({[(2S)-1-(4-amino-2-oxopyrimidin-1(2H)-yl)-3-hydroxypropan-2-yl]oxy}methyl)phosphonic acid | C8 H14 N3 O6 P | 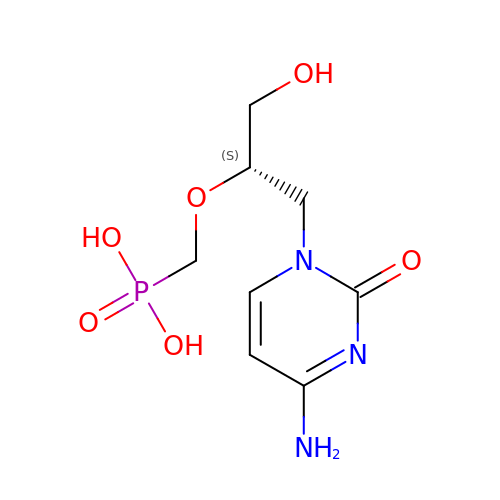VWFCHDSQECPREK-LURJTMIESA-N>[2x]MHHHHHHSTATNPLDLDVCAREPIHIPGLIQPYGVLLVIDPADGRIVQASTTAADLLGVPMAALLGMPYTQVLTLPEAQPFAVDDQPQHLMHAEVRFPQRATPPASAWVAAWHLYPQQWLVEMEPRDARLLDVTLREAMPLLRSVERDPGIAEAAVRVAKGLRSLIGFDRVMIYRFDEE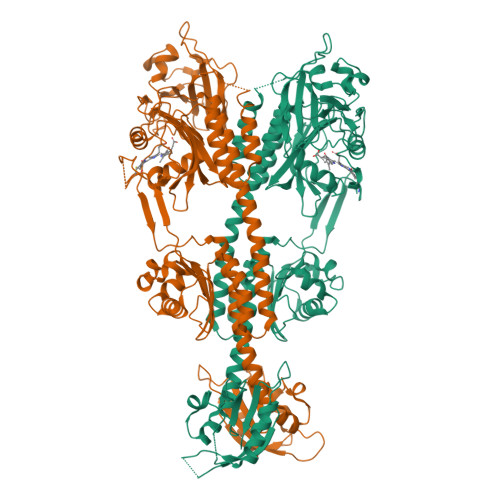WNGDIIAEARKPELEAYLGNHYPASDIPAQARALYLRNRVRQIADVGYQPSPIQPTVHPQLGTPVDLSDVSLRSVSPVHLEYLANMGVTATLVASIVVNDALWGLISCHHYSPHFTNHAMRDVTDAVARTLAGRIGALQAVARARLESVLLTVREKLITDFNDAEHMTVELLDDMAPDLMDVVDADGVAIFHGNDISRHGTTPDVAALRRIRDHIESEHHEALREDAVGALHVDAIGEVFPELADLAPLAAGFIFVPLMPQSRSALLWTRREQIQQIKWAGNPQLAKLEDIPNSRLSPRKSFDLWQQTVRGRARRWSPLHLESARSLRVLIELMERKRFQQDFTLLEASLSRLRDGVAIIERGTANAAHRLLFVNTAFADVCGSDVAELIGRELQTLYASDAPRANVELLQDALRNGRAAYVTLPLQVSDGAPVYRQFHLEPLPSPSGVTAHWLLQLRDPE>SGRPMFAVAVNEFIRSAGQDSLCGVPDINSSGDFMPLHIIVKEVPKVLPCCRRPKIKRTPYTLNDILDEPCPNQLKSSDLVTFTEPLVSNVKASSSIGLQILKHFDSGAKGSKNFITSASLGTVVKAETIDITKVLAKVRTAKAKVENDLVSRVMKTKRLCLGLVVETACVAAAGKLTEADNWEISGHTNANIGEAVVTATAELDKNLSRKIEIPPGTALAYSFMDLEILEDRSLRVSSSAGAMFDSGKAESTV[88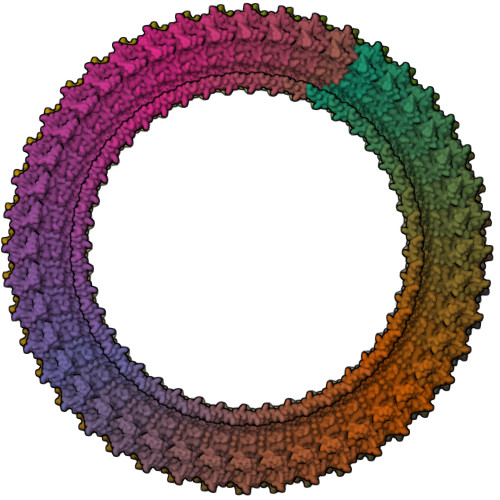x]> KVVKFSYMWTINNFSFCREEMGEVIKSSTFSSGANDKLKWCLRVNPKGLDEESKDYLSLYLLLVSCPKSEVRAKFKFSILNAKGEETKAMESQRAYRFVQGKDWGFKKFIRRDFLLDEANGLLPDDKLTLFCEVSVVQD;> NDDDVQKADVSSTGQGV

The adaptor protein, speckle-type BTB/POZ protein (SPOP), recruits substrates to the cullin-3-subclass of E3 ligase for selective protein ubiquitylation. SPOP recruits substrates via its N-terminal MATH domain, whereas a central BTB domain mediates dimerization and interactions with Cul3. Here, we show that MyD88 interacts with SPOP through a long degron that contains the established SPOP-binding consensus and an N-terminal site that we name the Q-motif. We determine the structural basis of these interactions and show that the Q-motif interacts with an unexplored binding pocket on the SPOP MATH domain.

We found that the search motif is present in six additional known SPOP substrates – GLI family zinc finger 2 (GLI2), DEK, steroid receptor coactivator-3 (SRC-3; also known as nuclear receptor coactivator 3 (NCoA-3)), sentrin-specific protease 7 (SENP7), SET domain-containing protein 2 (SETD2), and Caprin1. We crystallized SPOPMATH in complex with the 17-mer substrate peptides and obtained high-resolution structures of SPOPMATH in complex with SRC-3, SETD2, and Caprin1. The SRC-3, SETD2, and Caprin1 peptides all interact at the SPOPMATH substrate-binding groove with the same overall backbone conformation as MyD88. In the N-terminal region, the backbone atoms of peptide positions −3,–5, and −6 make identical hydrogen-bond contacts with main chain atoms of SPOP Lys135 and Arg138 and with the side chain of SPOP Tyr83, respectively. At the −4 position, the SRC-3, SETD2, and Caprin1 peptides all contain a glutamine residue corresponding to MyD88 Gln130, and the side chain of this residue makes identical contacts with the backbone carbonyl groups of SPOP Lys115 and Tyr136. The SPOPMATH hydrophobic pocket (SPOP Phe136, Ile137, and Phe141) encompasses the side chains of peptide positions −4 and −5. The SBC regions of the SRC-3, SETD2, and Caprin1 peptides also interact with SPOPMATH as reported in other substrates, with the exception of the SETD2 and SRC-3 residues that deviate from the consensus at the +4 and +5 positions, respectively. The 17-mer peptides of Caprin1, GLI2, and SRC-3 bound with the highest affinity, whereas the DEK peptides had the lowest-affinity interactions, with little difference between the 17-mer and 9-mer peptides. In cells, we confirmed the interaction of endogenous SPOP to overexpressed Caprin1, SENP7, and SRC-3 by coimmunoprecipitation in HEK293T cells. Similar to MyD88, mutation of the Q-motif abolished the interactions, consistent with the finding that the Q-motif is necessary for interaction of SPOP to these proteins.>[2x]GAMGSFNSIDVEINMYPVNKTSCNSSIGSSSTISTSELTITLTHEDCTPVFIGDYYSVVDKLATSGFFTNDKVHQDLTTQCKINLE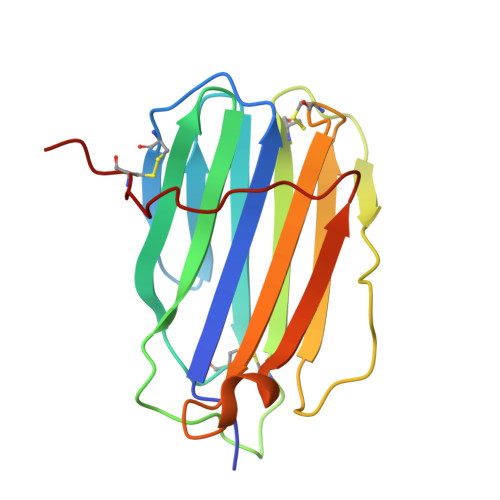IKCNSGRESRQLTPTTKVYLMPHSETVTVVGDCLSNLDVYIVYANTDAIYSDMDVVAYHTSYILNVDHIPPNDCERD> MARSQLSAAGEQHVIQLNQQGGKNLFCFPPISGFGIYFKDLALQLNHKAAVYGFHFIEEDSRIEQYVSRITEIQPE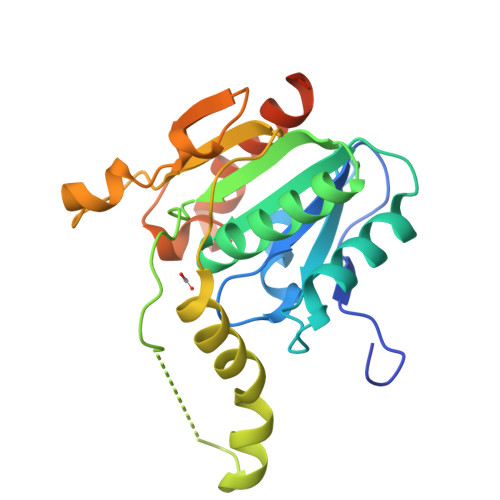GPYVLLGYSAGGNLAFEVVQAMEQKGLEVSDFIIVDAYKKDQSITADTENDDSAAYLPEAVRETVMQKKRCYQEYWAQLINEGRIKSNIHFIEAGIQTETSGAMVLQKWQDAAEEGYAEYTGYGAHKDMLEGEFAEKNANIILNILDKINSDQKVLPNKHGSHHHHHH> MGVPFFSSLRCMVDLGPCWAGGLTAEMKLLLALAGLLAILATPQPSEGAAPAVLGEVDTSLVLSSMEEAKQLVDKAYKERRESIKQRLRSGSASPMELLSYFKQPVAATRTAVRAADYLHVALDLLERKLRSLWRRPFNVTDVLTPAQLNVLSKSSGCAYQDVGVTCPEQDKYRTITGMCNNRRSPTLGASNRAFVRWLPAEYEDGFSLPYGWTPGVKRNGFPVALARAVSNEIVRFPTDQLTPDQERSLMFMQWGQLLDHDLDFTPEPAARASFVTGVNCETSCVQQPPCFPLKIPPNDPRIKNQADCIPFFRSCPACPGSNITIRNQINALTSFVDASMVYGSEEPLARNLRNMSNQLGLLAVNQRFQDNGRALLPFDNLHDDPCLLTNRSARIPCFLAGDTRSSEMPELTSMHTLLLREHNRLATELKSLNPRWDGERLYQEARKIVGAMVQIITYRDYLPLVLGPTAMRKYLPTYRSYNDSVDPRIANVFTNAFRYGHTLIQPFMFRLDNRYQPMEPNPRVPLSRVFFASWRVVLEGGIDPILRGLMATPAKLNRQNQIAVDEIRERLFEQVMRIGLDLPALNMQRSRDHGLPGYNAWRRFCGLPQPETVGQLGTVLRNLKLARKLMEQYGTPNNIDIWMGGVSEPLKR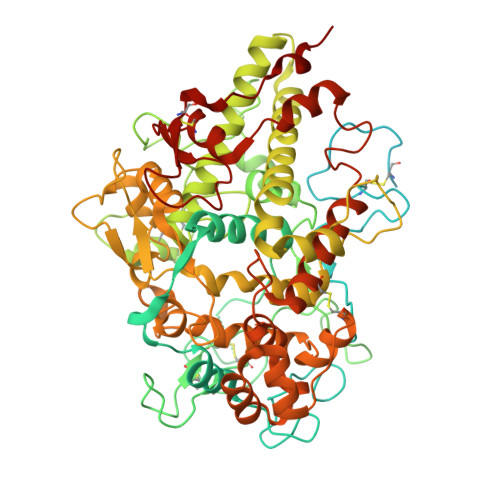KGRVGPLLACIIGTQFRKLRDGDRFWWENEGVFSMQQRQALAQISLPRIICDNTGITTVSKNNIFMSNSYPRDFVNCSTLPALNLASWREAS>[6x]PIFTLNTNIKATDVPSDFLSSTSALVGNILSKPGSYVAVHINTDQQLSF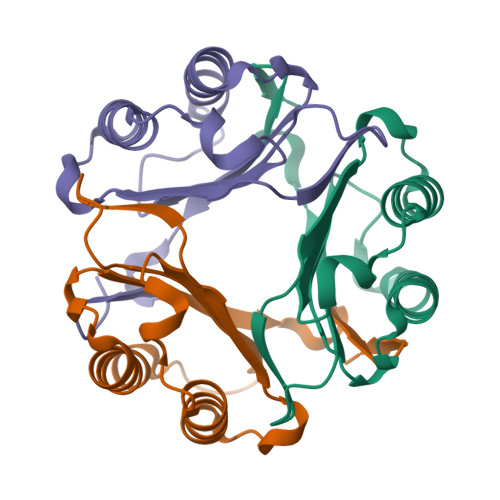GGSTNPAAFGTLMSIGGIEPSRNRDHSAKLFDHLNTKLGIPKNRMYIHFVNLNGDDVGWNGTTF> MASKYAVKLQTDFDNPKWIKRHKFMFDYLDINGNGQITLDEIVSKASDDICKNLGATPAQTQRHQDCVEAFFRGCGLEYGKETKFPEFLEGWKNLANADLAKWARNEPTLIREWGDAVFDIFDKDGSGTITLDEWKAYGRISGISPSEEDCEKTFQHCDLDNSGELDVDEMTRQHLGFWYTLDPE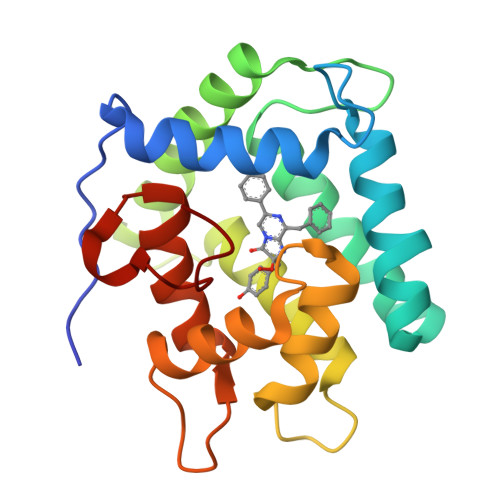ADGLYGNGVP In this study, the flax cytosolic cytokinin oxidase/dehydrogenase LuCKX1.1, an enzyme involved in the irreversible degradation of hormones in the cytokinin family, was identified as a potential virulence target of the flax rust effector AvrL567‐A. Cytokinins are responsible for the regulation of cell division and plant development, and have also been implicated in plant immunity. We investigated the interactions between AvrL567‐A and LuCKX1.1, and demonstrated that AvrL567‐A increases the enzymatic activity of LuCKX1.1 in vitro. The crystal structure of LuCKX1.1 was determined, providing insights into the molecular basis of the LuCKX1–AvrL567‐A interaction and the action of the effector on LuCKX1.1 enzymatic activity. The results indicated that LuCKX1.1 preferentially catalyses the oxidative cleavage of 2iP and tZ over the aromatic cytokinin types BA or kinetin.

To obtain insights into the molecular basis of the AvrL567‐A–LuCKX1.1 interaction, the flax LuCKX1.1 protein (residues 44–534) was crystallized. The final refined model of LuCKX1.1 contains residues 44–532. The structure of LuCKX1.1 exhibits a two‐domain topology consisting of a flavin adenine dinucleotide (FAD)‐binding domain and a substrate‐binding domain, which is similar to the known structures of AtCKX7, ZmCKX1, ZmCKX2, ZmCKX4a and ZmCKX4b. LuCKX1.1 contains the FAD co‐factor covalently linked to histidine‐104 (His104) via the 8‐methyl group of the flavin ring in LuCKX1.1. The FAD‐binding domain (residues 44–243 and 478–532) comprises one mixed β‐sheet, one antiparallel β‐sheet and flanking α‐helices. The other domain (residues 244–477) contains an antiparallel β‐sheet surrounded by α‐helices. The residues important for substrate binding identified in the active sites of ZmCKX1 and ZmCKX2 are largely conserved in LuCKX1.1, including aspartic acid‐168 (Asp168), glutamic acid‐281 (Glu281), valine‐365 (Val365), glutamic acid‐369 (Glu369), tryptophan‐384 (Trp384), proline‐413 (Pro413), leucine‐446 (Leu446) and leucine‐483 (Leu483). The iA1.1 clone initially isolated by Y2H screening encodes residues 268–340 of LuCKX1.1, indicating that these 72 residues are sufficient for the interaction with AvrL567‐A. In the crystal structure, this fragment corresponds to two buried β‐strands and two surface‐exposed regions of helices and loops. Surface 1 is right above the opening of the channel through which cytokinins enter the active site. In the high‐resolution crystal structure of LuCKX1.1, the electron density map for the surface 1 region is not well resolved, indicating flexibility in this loop region.

>[2x]SLDLQGSIDYSTLAAGKDFGGVYSSNPLALIRPSGADDVARVLKSACRSSNLTVAARGNGHSINGQAMADGGIVLDMRSTEGNHFKILRINGGDHYADVSGGALWEDILMRCVSEYGLAPRSWTDYLRLTVGGTLSNAGVSGQAFRYGPQSSNVTELDVVTGKGDFLTCSPTQNSDLFFGALGGLGQFGVITRARIPLEPAPDMVRWIRMVYAEFEDFSRDAEWLVTQPEKESFDYVEGFAFVNSDSPADGWPSVPLNHMMTTPIHSGHQLLYCLELALHFNHSNSSSTVDSVVKRLIGGLRYMKGFKYEVDLSYVEFVMRVKRVEEDARAHGMWDAPHPWLNLFVSKADIAEFDRLIFKGLLHDGVGGPMLVYPLLRSKWDSRSSVVLPEGEDEIFYIVALLRSNPPYPKGPSVDKLVSQNDKIIQSCIQHGLGFKLYLPHYQSQHDWRRHFGDQWSKFVQLKLAFDPMAVLAPGQKIFTRRTKKDPA Nalpha-(tert-butoxycarbonyl)-N-1H-tetrazol-5-yl-D-tryptophanamide 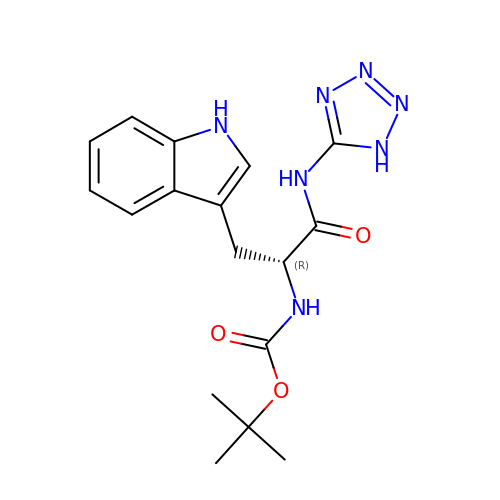| C17 H21 N7 O3 | OGAGNLWYSIOVOG-CYBMUJFWSA-N CT and LT, with their five equivalent binding subunits, are known to be multivalent proteins. Binding has been described as a “two-fingered grip”, provided by the two terminal residues, galactose (Gal) and sialic acid (NeuAc). The specificity of this interaction is mainly determined by the terminal galactose residue, which is buried in a deep pocket at the rugged underside of the toxin (distant from the A-subunit). As expected, all three inhibitors bind in the primary binding site, acting as decoys for the toxins’ main receptor, the GM1 ganglioside.

Compounds 2 and 3 are bidentate ligands that combine the two terminal residues of the GM1 oligosaccharide, i.e. galactose and sialic acid. The cholera toxins come in two varieties: classical (c) and El Tor (ET). The two biotypes differ at two amino acid residues in the B-subunit, 18 and 47 (His18 and Thr47 in cCTB, and Tyr18 and Ile47 in ET CTB). The crystal structures were solved to 1.1 Å resolution and contain one B-pentamer in the asymmetric unit. Both CT variants have well-defined electron density for inhibitor 2 in all binding sites. As in the other structures, the galactose moiety of 2 is buried in the GM1 binding site, H-bonding with Glu51, Gln61, Asn90 and Lys91. The sialic acid residue has direct interactions with the backbones of Glu11 and His13. The differences to GM1-os binding can be seen in the linker region of 2, where the hydrogen bond of the core Gal to the side chain of His13 is no longer achievable. Instead, closer to the terminal Gal, the carbonyl group of the linker engages in a water-mediated interaction to Asn14.

>TPQNITDLCAEYHNTQIHTLNDKIFSYTESLAGKREMAIITFKNGATFQVEVPGSQHIDSQKKAIERMKDTLRIAYLTEAKVEKLCVWNNKTPHAIAAISMAN[5x]>[4x]MKETNSEEADSGLAFFRNMYDKYRDAFLSHLNEYSLEEEIKE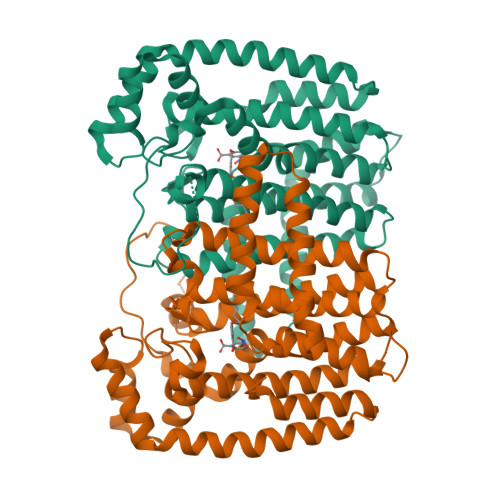HISKYYKLLFDYNCLGGKNNRGILVILIYEYVKNRDINSSEWEKAACLAWCIEILQAAFLVADDIMDKGEMRRNKYCWYLLKDVETKNAVNDVLLLYNSIYKLIEIYLRNESCYVDVIATFRDATLKTIIGQHLDTNIFSDKYSDAHREIDVNNINVPEQPVIDINMINFGVYKNIVIHKTAYYSFFLPIVCGMLLAGIAVDNLIYKKIEDISMLMGEYFQIHDDYLDIFGDSTKTGKVGSDIQNNKLTWPLIKTFELCSEPDKIKIVKNYGKNNLACVKVIDSLYEQYKIRKHYESYEKAQKAKILSAINELHHEGIEYVLKYLLEILFTGV> MRLLKYPL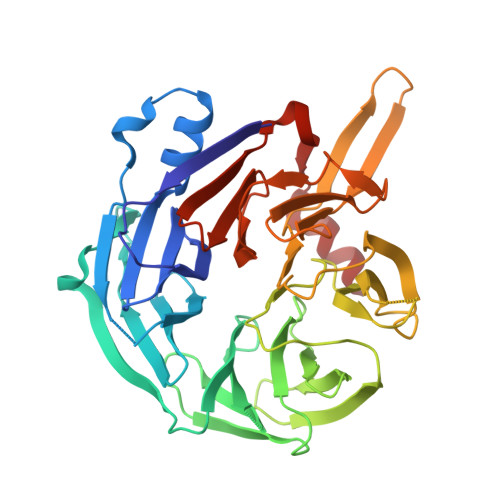DIHNEQVNALAALGPYIILAGSGGHVMAWRQQQLVDTAFDRVMIKDLKPEVSFQVDQDTTGDIFFITGDLETLYIGSEHRLWGYSGWLCRDTNNINSVEKMNSKLLFECKSPSTITDVKYDINLGILFVLLSNENKILLFRHKTFDKLSEITIDKASKPITGIIDPTGQTFTVMTSDRSILVYQINKTGTHKLINKLTQHVQMYPLHYRISMSPQADILPVINSVKGVPNNATSCTALLDRNNNYKVTKTLVTPSSNGCRVLVYSPAFYEKPNLKKGTSTRYNLIATSGSTDGTILVWNTKRMKPLFNALQVSSTAINDMSWSQDGFTLFAISNDATLYTFAFQEKDLGVALPQTEIKSLQEVNK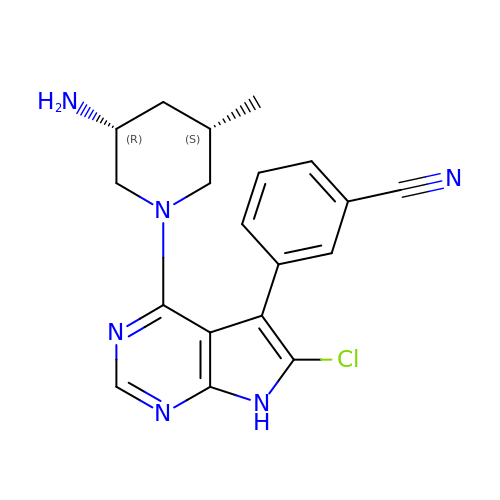(3P)-3-{4-[(3R,5S)-3-amino-5-methylpiperidin-1-yl]-6-chloro-7H-pyrrolo[2,3-d]pyrimidin-5-yl}benzonitrile | C19 H19 Cl N6 | BSBZFPBEYMSVPJ-SMDDNHRTSA-N> R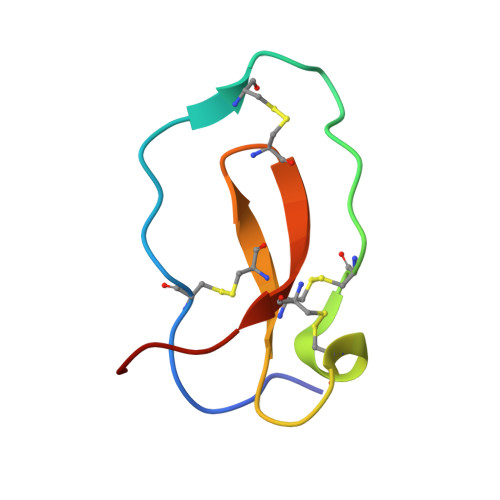RKPGKCPVTYGQCLMLNPPNFCEMDGQCKRDLKCCMGMCGKSCVSPVKA> PPAIPGIPGIP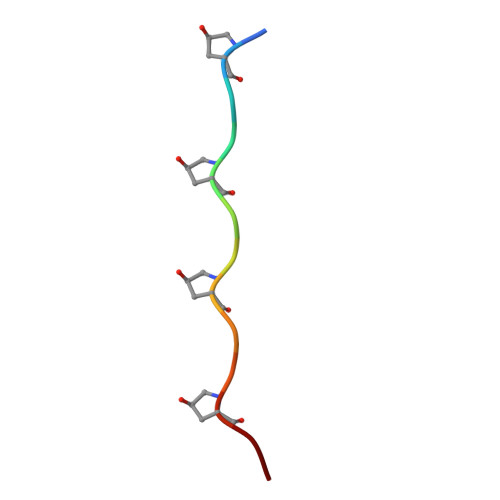GT5'-O-{[(2S,3R)-2,3-diaminobutanoyl]sulfamoyl}adenosine | C14 H22 N8 O7 S | 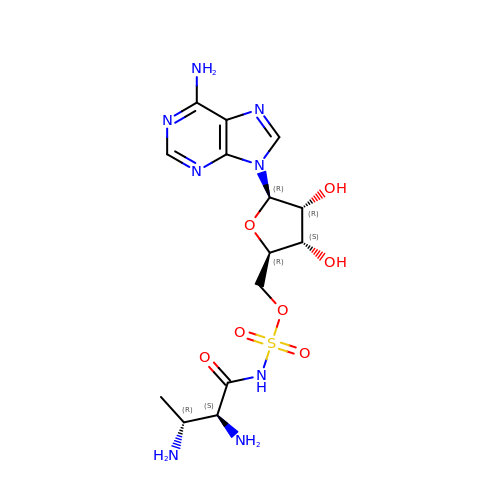MASQMYRALSQMDU-CKTDUXNWSA-N> MQSTSNHLWLLSDILGQGATANVFRGRHKKTGDLFAIKVFNNISFLRPVDVQMREFEVLKKLNHKNIVKLFAIEEETTTRHKVLIMEFCPCGSLYTVLEEPSNAYGLPESEFLIVLRDVVGGMNHLRENGIVHRNIKPGNIMRVIGEDGQSVYKLTDFGAARELEDDEQFVSLYGTEEYLHPDMYERAVLRKDHQKKYGATVDLWSIGVTFYHAATGSLPFRPFEGPRRNKEVMYKIITGKPSGAISGVQKAENGPIDWSGDMPVSCSLSRGLQVLLTPVLANILEADQEKCWGFDQFFAETSDILHRMVIHVFSLQQMTAHKIYIHSYNTATIFHELVYKQTKIISSNQELIYEGRRLVLEPGRLAQHFPKTTEENPIFVVSREPLNTIGLIYEKISLPKVHPRYDLDGDASMAKAITGVVCYACRIASTLLLYQELMRKGIRWLIELIKDDYNETVHKKTEVVITLDFCIRNIEKTVKVYEKLMKINLEAAELGEISDIHTKLLRLSSSQGTIETSLQDIDSRLSPGGSLADAWAHQEGTHPKDRNVEKLQVLLNCMTEIYYQFKKDKAERRLAYNEEQIHKFDKQKLYYHATKAMTHFTDECVKKYEAFLNKSEEWIRKMLHLRKQLLSLTNQCFDIEEEVSKYQEYTNELQETLPQKMFTASSGIKHTMTPIYPSSNTLVEMTLGMKKLKEEMEGVVKELAENNHILERFGSLTMDGGLRNVDCLGIHR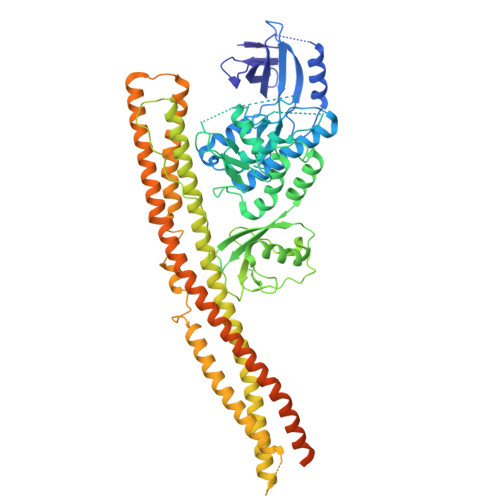PDYKDDDDK> SSQIRQNYSTEVEAAVNRLVNLYLRASYTYLSLGFYFDRDDVALEGVCHFFRELAEEKREGAERLLKMQNQRGGRALFQDLQKPSQDEWGTTLDAMKAAIVLEKSLNQALLDLHALGSAQADPHLCDFLESHFLDEEVKLIKKMGDHLTNIQRLVGSQAGLGEYLFERLTLKHD

Auranofin (AF), a gold(I) compound that is currently used for the treatment of rheumatoid arthritis and is in clinical trials for its promising anticancer activity, was encapsulated within the human H-chain and the horse spleen ferritin nanocages using the alkaline disassembly/reassembly protocol. Mammalian Fts are composed of two different chains, the H-chain (heavy) and the L-chain (light), that assemble to form a hollow cage-like structure with an internal diameter of 8 nm and an external one of 12 nm. In particular, two different ferritins were selected for this kind of study: the human H-chain ferritin (hHFt) and the horse spleen ferritin (hsFt), which is mainly L-chain. In fact, in both AFhsFt and AFhHFt structures, the gold atoms are found close to the side chains of cysteine residues.

At variance with what was observed for AFhHFt, the structure of AFhsFt presented a single gold binding site. A gold atom with 0.20 occupancy binds the SG atom of Cys126; a water molecule completes the metal coordination sphere, giving rise to a linear geometry. In the structure of AFhsFt, a gold atom is bound to Cys126, buried at the interface between two hsFt subunits. The gold binding site close to Cys126 is not surprising since it has been already observed in the X-ray structures of other gold-encapsulated hsFts. ICP-AES data indicated that about 270 gold atoms were encapsulated within AFhsFt, achieving a protein chain to metallodrug molar ratio of ~1:11, while only about 90 atoms of gold were found in the nanocage based on the human H-chain Ft, with a protein chain to metallodrug molar ratio of ~1:4. In the case of AFhsFt, the comparison between the structural data and the ICP-AES results (one gold binding site in the X-ray structure and 11 AF molecules per hsFt chain suggested via ICP-AES data) demonstrated that a significant fraction of AF is not directly bound to the protein, but it is encapsulated in the bulk of the hsFt nanocage. Considering that 270 molecules of AF are encapsulated within hsFt and just one gold binding site has been identified on the AFhsFt structure, it can be concluded that many loaded AF molecules are trapped within the bulk. This suggests that AFhsFt has a high number of AF molecules that can be released from its bulk and that it preserves the features of the native protein and thus its ability to be recognized by the Scara5 receptor. On the contrary, AFhsFt preserved almost the same cytotoxicity of AF on the cancer cell line, but its selectivity was also decreased when compared to free AF.>MAGVRLVDVWKVFGEVTAVREMSLEVKDGEFMILLGPSGCGKTTTLRMIAGLEEPSRGQIYIGDKLVADPEKGIFVPPKDRDIAMVFQSYALYPHMTVYDNIAFPLKLRKVPRQEIDQRVREVAELLGLTELLNRKPRELSGGQRQRVALGRAIVRKPQVFLMDEPLSNLDAKLRVRMRAELKKLQRQLGVTTIYVTH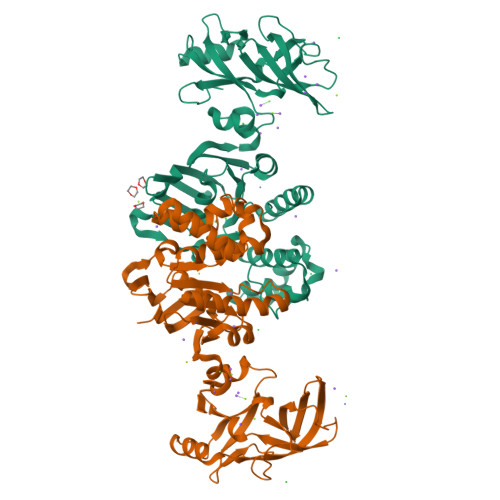DQVEAMTMGDRIAVMNRGVLQQVGSPDEVYDKPANTFVAGFIGSPPMNFLDAIVTEDGFVDFGEFRLKLLPDQFEVLGELGYVGREVIFGIRPEDLYDAMFAQVRVPGENLVRAVVEIVENLGSERIVRLRVGGVTFVGSFRSESRVREGVEVDVVFDMKKIHIFDKTTGKAIF[2x]>MAVVFVNKLTLIGDAEEFESRYEAVGAFMETQPGLVRYSLVRSTKDDSVYFNIAEWDDEDTFRKALAEPEFRRRLDALTGLIKGEPHLSLPVRQGRAAQVLENLYFQGHHHHHH[2x]

Rishirilides are a group of PKS II secondary metabolites produced by Streptomyces bottropensis Gö C4/4. Structurally, rishirilide is a tricyclic partially aromatic polyketide with an unusual isopentyl sidechain and a carbonyl group on the third ring. In this study the involvement of one cyclase and two oxygenase in rishirilide biosynthesis was investigated. For this purpose, excision of rslC3 gene using the markerless time-saving CRISPR-Cas9 system, inactivation of rslO4 gene using Redirect® technology, and crystallization of RslO4 and RslO1 proteins were carried out.

The monooxygenase RslO4 crystallizes as a homodimer and the overall structure of each subunit is made up of three α-helices (α1–α3) and four β-strands (β1–β4) with a ferredoxin-like fold. The additional α-helix in the C-terminus of each monomer is generated by the TEV protease cleavage site of the His-tag sequence, which is required for protein purification. The three α-helices are located on one side of the homodimer. Together with an additional β-strand of the other subunit, a five-stranded antiparallel β-sheet, which is stabilized by ten main-chain hydrogen bonds between β2 and β4 of two chains. The interface between the two monomers is further stabilized by hydrophobic interactions provided by β-sheets and side chain hydrogen bonds contributed by Lys8, Ser43, Glu85 and His87. The closest structural homologue is SnoaB from S. nogalater, with a sequence identity of 41%. Closer inspection of the active site of RslO4 revealed high similarity between the positioning of Asn7, Asn52 and Trp56, which are represented by Asn18, Asn63 and Trp67 in SnoaB coordinating oxidized dithranol by hydrogen bonds. The high similarity of RslO4 in the sequence and three-dimensional structure with the monooxygenase SnoaB suggests that RslO4 mediates a mono-oxygenation in rishirilide biosynthetic pathway. Unlike SnoaB which oxygenates the middle non-aromatic ring of 12-deoxynogalonic acid during nogalomycin biosynthesis, RslO4 might oxygenate the third lateral aromatic ring in its tricyclic aromatic substrate to form a quinonic product. According to the observation from molecular dynamics simulations, Trp56 contributes in the orientation of substrate positioning inside RslO4 pocket through an H-Bonding network with the three –OH groups, which in turn leads to an electron delocalization in the third aromatic ring. The results of dynamic simulations match those of the Site-Directed Mutagenesis which demonstrated the importance of Asn7, Asn52, Trp56, Tyr22, and Met29 in the catalytic mechanism of RslO4.> MAHHHHHHMTAATDPLISLSHYYLPVYKPRQVVLERGQGARVWDSQGREFIDLAAGIAVCGLGHNDPD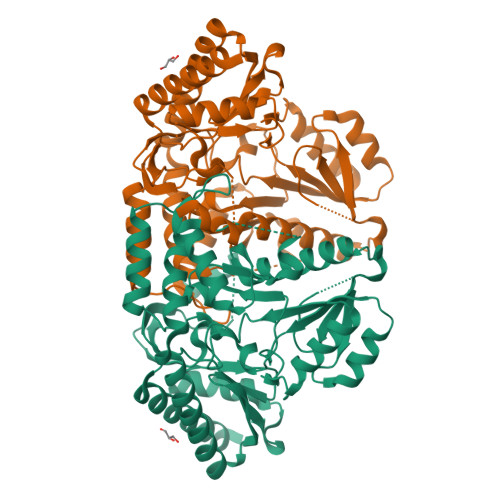LVAALVEQAGKLWHTSNVFYSAPPLHLAEELVKASRFAERVFLCNSGAEANEVAIKMVRKWASSQGRPADKRVIITFRGSFHGRTMGAVTATAQPKYQEGYEPLPGGFRYIDFNDEVQLETAMAAGDVAAVMLEPIQGEGGVMPAKSGFLKRVRELCDQHDALLVLDEIQAGMGRTGTLFAHWQDDVVPDMVTLAKALGGGFPIGAMLAGPKVAETMQFGAHGTTFGGNPLAAAVARVALRKLASSEIAANVSRQSKALRDGFARINEEFGVFSEVRGRGLMLGAVLSKDFAGQAGAILDHAAGQGLLTLQAGPDVLRFVPSLNITDEEVAEGLKRLRAAIAAFIAAR> MNKSRQKELTRWLKQQSVISQRWLNISRLLGFVSGILIIAQAWFMARILQHMIMENIPREALLLPFTLLVLTFVLRAWVVWLRERVGYHAGQHIRFAIRRQVLDRLQQAGPAWIQGKPAGSWATLVLEQIDDMHDYYARYLPQMALAVSVPLLIVVAIFPSNWAAALILLGTAPLIPLFMALVGMGAADANRRNFLALARLSGHFLDRLRGMETLRIFGRGEAEIESIRSASEDFRQRTMEVLRLAFLSSGILEFFTSLSIALVAVYFGFSYLGELDFGHYDTGVTLAAGFLALILAPEFFQPLRDLGTFYHAKAQAVGAADSLKTFMETPLAHPQRGEA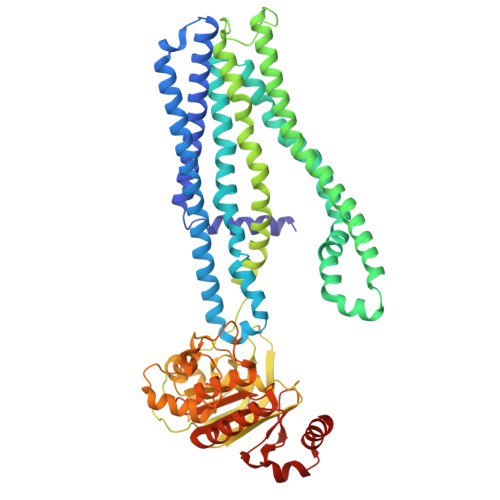ELASTDPVTIEAEELFITSPEGKTLAGPLNFTLPAGQRAVLVGRSGSGKSSLLNALSGFLSYQGSLRINGIELRDLSPESWRKHLSWVGQNPQLPAATLRDNVLLARPDASEQELQAALDNAWVSEFLPLLPQGVDTPVGDQAARLSVGQAQRVAVARALLNPCSLLLLDEPAASLDAHSEQRVMEALNAASLRQTTLMVTHQLEDLADWDVIWVMQDGRIIEQGRYAELSVAGGPFATLLAHRQEEI> MGNKSDAAAKQIKKLEEDFDGRIGVFAIDTGSGNTFGYRSDERFPLCSSFKGFLAAAVLERVQQKKLDINQKVK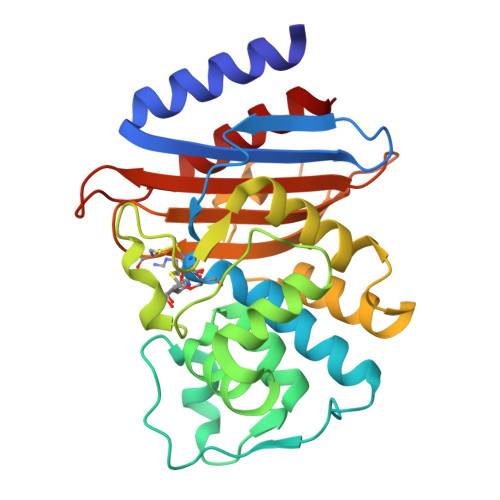YESRDLEYHSPITTKYKGSGMTLGDMASAALQYSDNGATNIIMERFLGGPEGMTKFMRSIGDNEFRLDRWALELNTAIPGDKRDTSTPKAVANSLNKLALGNVLNAKVKAIYQNWLKGNTTGDARIRASVPADWVVGDKTGSCGAYGTANDYAVIWPKNRAPLIVSIYTTRKSKDDKHSDKTIAEASRIAIQAID Escherichia coli phage SU10 belongs to the genus Kuravirus from the class Caudoviricetes of phages with short non-contractile tails. Here we show that the virion of SU10 has a prolate head, containing genome and ejection proteins, and a tail, which is formed of portal, adaptor, nozzle, and tail needle proteins and decorated with long and short fibers. In contrast to other short-tailed phages, the tails of Kuraviruses elongate upon cell attachment. After binding to the host, SU10 tail, nozzle proteins, and short fibers re-arrange to form a nozzle that extends the tail.

The dodecamer of SU10 adaptor proteins forms the interface between the dodecamer of portal proteins and hexamer of nozzle proteins. Six long tail fibers are attached to the sides of the adaptor complex. The coiled-coiled part of each long tail fiber is held by fiber dock loops from two neighboring adaptor proteins. The hexamer of nozzle proteins, attached to the adaptor, is decorated with six short tail fibers, and its central channel is plugged with a tail needle. In the SU10 virion, the Ig-like nozzle domains are organized into an L-shape arrangement. The first two nozzle domains form a blunt tip of the tail, then there is an 82° turn and the remaining two domains point towards the capsid. Nozzle domain 4 interacts with the short tail fiber dock loop from the nozzle protein located counterclockwise. The short tail fiber is attached to a fiber dock loop from a nozzle protein. The fiber dock loop contains tryptophans 839, 847, and 857, the side chains of which are arranged in a pseudo-threefold symmetry. The position of the short tail fiber is additionally stabilized by the interaction of the central domain of the short tail fiber with residues 71–78 of the long tail fiber.

>[2x]MAMPDVQYPINTYGWLKKAVALWADRDDDEFVNQIPNFINFAEKEIYRNLRIPPLEKEVYLDIKDGVAYIPPDYLEAQWMMRAKDGTIFQVTSPEEISYRRQHGTINPSHWNNQPVNFARFGSRFIFYPSIEADTPYYPDDGSPLIPAENSVILSYYADPPEFHEDTDTSTILTIAPELLLYFTLRHACLFVQDDNGVQKWSALGKAILDEMVEQNKKQEYSGSPIAIPNNMTRLQSSLPDIYGIRTSRV;>[3x]MAIETNAVVITDLNPLYPRDRDYIYEGAAQIRLIKQTLQNTFPNVTEPVDIDSDTFKIMSEKLKFTGDAMDVGGLMIKNVTPGTGDKDVVTKGQMEAFMKNWMENKLYRIGSYYITEEDINPGDSISLGFGSWAKVTGVIMGTGVVNPDGSVPNAQRVEFQAGGTGGRVFNTIRTENVPLMTVNGSSFSLSSNTHSHNMVFGRGDASGHNSSPNWYSPGGGYSQRTDNDTHTHTISGSVSLGRDDISRQPINTLPPFRAAHIWRRIS;>MIVYNNQAPDAVNNVGQFGATEGSIGAYKQAAEYAADSKYWALLAESKFGTIDDLIAEVERLYQQGVLMKQDIEDLKQDFKDQDARLMSLIAQTNAAVSDANNAVALINQKLIEVQNQLDVLLGMSVDVTTLPPGTPATGSFNPNTGVISLGIPEGEPGKDGSVKDLDTAPTGVPELGDLGFYVDKDDNTVHKTTLENIANLTPSVRSVSVNGGPALDGEVALTINKETVGLGNVLNVAQYSRQEINDKFDKTTKTYQSKAEAYADAQYRQVGEKVLVWEATKYEFYTVAANKTLTPVKTEGRILTVNSRSPDSSGNIDITIPTGNPSLYLGEMVMFPYDPSKNISYPGVLPADGRLVSKESASDLGPSLVSGQLPVVSETEWQSGAKQYFSWGKLADGITDADSTNFINIRLPDWTGGEAIRAPDSDKDSQYNGSVQAQKPYVVTVNNQAPDEITGNVNISRSILGAASSGANSDITSLSGLTTPLSISQGGTGAKDAASARSNLGLGSVSTLDNVPIASGGTGAGDAAGARFNLGLGNSATMNTGTNSDNVLKVGDFGIGRPDGALVFDTTSQDQLLAGLDTYGLCVFRNNQQIAAPWDIWNYSSNLFFRAGDTYSMISIPFESAGKIKVFGGASGSGWKTSRTVYDTVNTTVDVNGFIKAASPIVKVFHDGSFETNEQSDGVSVKKISTGVYLISGCLGLNSDAGWGGVDGGFEIPIDRNKQPRVWLDYEVKEDGSLLIKTYHRTHSTSPAFARNELEGFSDGDPVDIPKDAFISVRVEMPSK[3x];> MALYPIKSLGAVGVIADQAPTDLAPNAFTNAINARFVEQRVFKTGGNAPLSYVDEDKDLTPLSFVSMPFDYYSAGNSFLVVGTNKKLYKLTDESLTDISRKVATVTKKASASIKIYPVVSQIVPKESTISMNFNQTKNLEVSLLPADANNTNLIWEVSNSSYGSITVDPSDSKLATLTSFEKEGNLVVTISTANESVVAQIAVNIIDGDSGIFLSQDTVTIRKGGTTTLTAVTGKTPVTWSSNNASIVSVTPNANSLTAVITANGEGNVTITADNGTKTASCEIVSIPQIDSISLSQSDVTVSRGSQYILTATLSPANAPNQNITWTSSNPNIATVSGTSTQGTINALLAGFTEITATTEEGNRVAVCTVRVDLAGRTMRTSAMAFAAPVSESVETQEEEVVTPPESEETVYFAEPTSGIDTSGMYEGNNFYDYSNVNDIEGFARASLLATPLSSVTLDIVSASLDVGEEIVITATASPEGEYSYQWSVDKTGYVSTTSVTGKSIKLVALRKGEINVTCTVSQMTQKDYDAFDDYPWYHAVISNCAVATTHYETPQVKEFESEYFVDLPGWGEQTVVDNDGNPSVKKFNWKCERVRSFNNRLFALNMREANASGVTTNYPLRLRWSNFANENKAPTLWDDFAYDRVVSSDLASNIVGQTQALENGYAGYIDLADSNGSLIDILPLKDYLFVYTEFETYIGSPTNNTYQPLMFKKLFNDSGILAPECVVEVEGSHFVVTQNDVILHNGATKKSIASNRVKNMLINEVCLVNPLATRVHLHQDKKEVWVLYVGPGEPKESFACTKAAVWNYEFDTWSFRTIPYAQCIGLVDPPVLERGPIWSDFQEITWDDPSIKELVWRKDATNFRQRVTIVGSFLKGFYQVDVGALDYFYDRLNDVVIEKPLEMRLERTGIDFDNVTNEWNQKHINRFRPQTTGSGTYIFEAGGSQFSNEYGHPHTSKTYTIGVDRHVSVRLNHPYLFYNVIDNDVNSNAAINGLTIEFAVGGRR> PAMLPISMSDEGDSFLVKDSLGENKIPKNPSKVVILDLGILDTFDALKLNDKVVGVPAKNLPKYLQQFKNKPSVGGVQQVDFEAINALKPDLIIISGRQSKFYDKL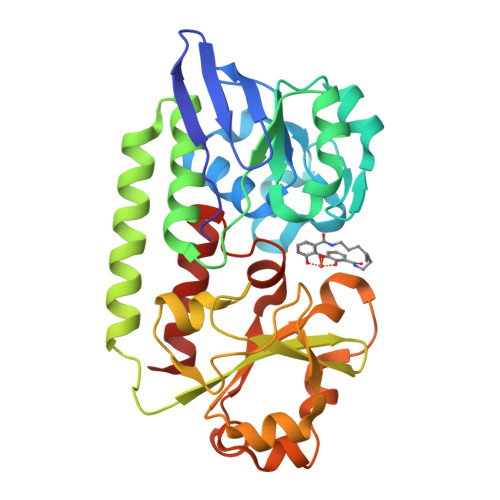KEIAPTLFVGLDNANFLSSFENNVLSVAKLYGLEKEALEKISDIKNEIEKAKSIVDEDKKALIILTNSNKISAFGPQSRFGIIHDVLGINAVDENIKVGTHGKSINSEFILEKNPDYIFVVDRNVILGNKERAQGILDNALVAKTKAAQNKKIIYLDPEYWYLASGNGLESLKTMILEIKNAVK5-AMINO-1,3,4-THIADIAZOLE-2-SULFONAMIDE | C2 H4 N4 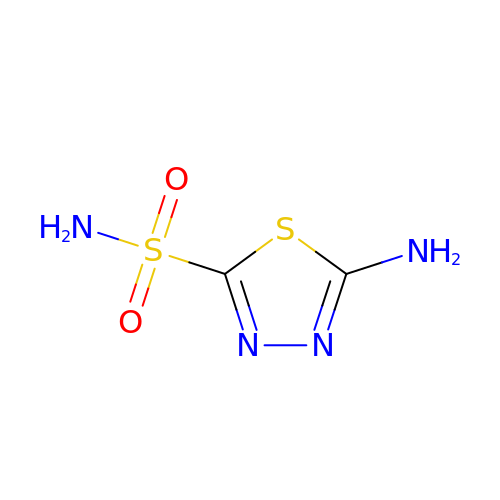O2 S2 | VGMVBPQOACUDRU-UHFFFAOYSA-N> FMVSLPRMVYPQPKVLTPCRKDVLVVTPWLAPIVWEGTFNIDILNEQFRLQNTTIGLT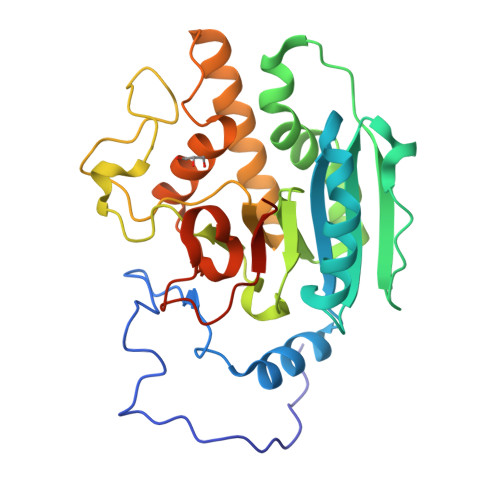VFAIKKYVAFLKLFLETAEKHFMVGHRVHYYVFTDQPAAVPRVTLGTGRQLSVLEVRAYKRWQDVSMRRMEMISDFCERRFLSEVDYLVCVDVDMEFRDHVGVEILTPLFGTLHPSFYGSSREAFTYERRPQSQAYIPKDEGDFYYMGAFFGGSVQEVQRLTRACHQAMMVDQANGIEAVWHDESHLNKYLLRHKPTKVLSPEYLWDQQLLGWPAVLRKLRFTAVPKNHQAVRNPE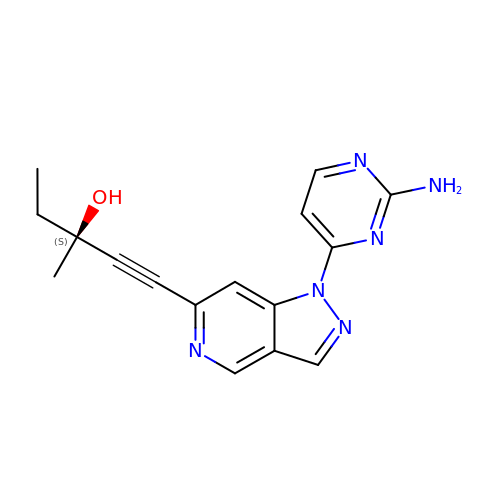(3S)-1-[1-(2-aminopyrimidin-4-yl)-1H-pyrazolo[4,3-c]pyridin-6-yl]-3-methylpent-1-yn-3-ol | C16 H16 N6 O | WZLQQYUWMGFXDE-INIZCTEOSA-N> MAFLRSMWGVLSALGRSGAELCTGCGSRLRSPFSFVYLPRWFSSVLASSPKKPVSSYLRFSKEQLPIFKAQNPDAKTTELIRRIAQRWRELPDSKKKIYQDAYRAEWQVYKEEISRFKEQLTPSQIMSLEKEIMDKHLKRKAMTKKKELTLLGKPKRPRSAYNVYVAERFQEAKGDSPQEKLKTVKENWKNLSDSEKELYIQHAKEDETRYHNEMKSWEEQMIEVGRKDLLRRTIKKQRKYGAEEC;> MWIPVVGLPRRLRLSALAGAGRFCILGSEAATRKHLPARNHCGLSDSSPQLWPEPDFRNPPRKASKASLDFKRYVTDRRLAETLAQIYLGKPSRPPHLLLECNPGPGILTQALLEAGAKVVALESDKTFIPHLESLGKNLDGKLRVIHCDFFKLDPRSGGVIKPPAMSSRGLFKNLGIEAVPWTADIPLKVVGMFPSRGEKRALWKLAYDLYSCTSIYKFGRIEVNMFIGEKEFQKLMADPGNPDLYHVLSVIWQLACEIKVLHMEPWSSFDIYTRKGPLENPKRRELLDQLQQKLYLIQMIPRQNLFTKNLTPMNYNIFFHLLKHCFGRRSATVIDHLRSLTPLDARDILMQIGKQEDEKVVNMHPQDFKTLFETIERSKDCAYKWLYDETLEDR;> MSALCWGRGAAGLKRALRPCGRPGLPGKEGTAGGVCGPRRSSSASPQEQDQDRRKDWGHVELLEVLQARVRQLQAESVSEVVVNRVDVARLPECGSGDGSLQPPRKVQMGAKDATPVPCGRWAKILEKDKRTQQMRMQRLKAKLQMPFQSGEFKALTRRLQVEPRLLSKQMAGCLEDCTRQAPESPWEEQLARLLQEAPGKLSLDVEQAPSGQHSQAQLSGQQQRLLAFFKCCLLTDQLPLAHHLLVVHHGQRQKRKLLTLDMYNAVMLGWARQGAFKELVYVLFMVKDAGLTPDLLSYAAALQCMGRQDQDAGTIERCLEQMSQEGLKLQALFTAVLLSEEDRATVLKAVHKVKPTFSLPPQLPPPVNTSKLLRDVYAKDGRVSYPKLHLPLKTLQCLFEKQLHMELASRVCVVSVEKPTLPSKEVKHARKTLKTLRDQWEKALCRALRETKNRLEREVYEGRFSLYPFLCLLDEREVVRMLLQVLQALPAQGESFTTLARELSARTFSRHVVQRQRVSGQVQALQNHYRKYLCLLASDAEVPEPCLPRQYWEELGAPEALREQPWPLPVQMELGKLLAEMLVQATQMPCSLDKPHRSSRLVPVLYHVYSFRNVQQIGILKPHPAYVQLLEKAAEPTLTFEAVDVPMLCPPLPWTSPHSGAFLLSPTKLMRTVEGATQHQELLETCPPTALHGALDALTQLGNCAWRVNGRVLDLVLQLFQAKGCPQLGVPAPPSEAPQPPEAHLPHSAAPARKAELRRELAHCQKVAREMHSLRAEALYRLSLAQHLRDRVFWLPHNMDFRGRTYPCPPHFNHLGSDVARALLEFAQGRPLGPHGLDWLKIHLVNLTGLKKREPLRKRLAFAEEVMDDILDSADQPLTGRKWWMGAEEPWQTLACCMEVANAVRASDPAAYVSHLPVHQDGSCNGLQHYAALGRDSVGAASVNLEPSDVPQDVYSGVAAQVEVFR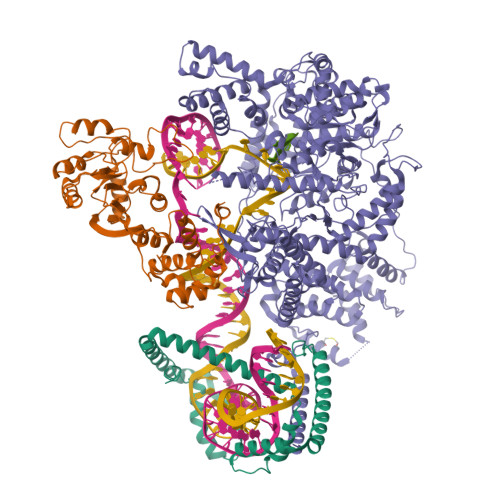RQDAQRGMRVAQVLEGFITRKVVKQTVMTVVYGVTRYGGRLQIEKRLRELSDFPQEFVWEASHYLVRQVFKSLQEMFSGTRAIQHWLTESARLISHMGSVVEWVTPLGVPVIQPYRLDSKVKQIGGGIQSITYTHNGDISRKPNTRKQKNGFPPNFIHSLDSSHMMLTALHCYRKGLTFVSVHDCYWTHAADVSVMNQVCREQFVRLHSEPILQDLSRFLVKRFCSEPQKILEASQLKETLQAVPKPGAFDLEQVKRSTYFFS> LDKVYQMKSKPRGYCLIINNHNFAKA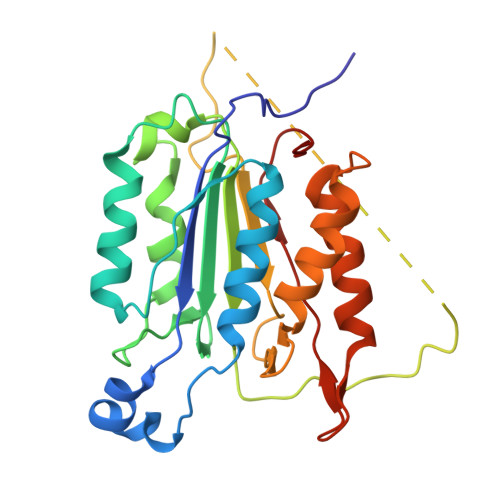REKVPKLHSIRDRNGTHLDAGALTTTFEELHFEIKPHHDCTVEQIYEILKIYQLMDHSNMDCFICCILSHGDKGIIYGTDGQEAPIYELTSQFTGLKCPSLAGKPKVFFIQACQGDNYQKGIPVETDSEEQPYLEMDLSSPQTRYIPDEADFLLGMATVNNCVSYRNPAEGTWYIQSLCQSLRERCPRGDDILTILTEVNYEVSNKDDKKNMGKQMPQPTFTLRKKLVFPSD> GAMGSYKDNIRHGVCWIYYPDGGSLVGEVNEDGEMTGEKIAYVYPDE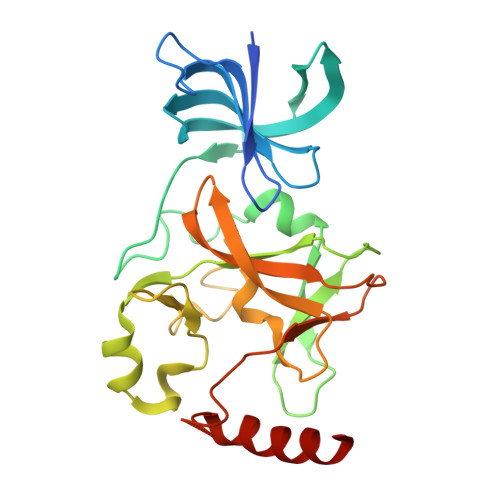RTALYGKFIDGEMIEGKLATLMSTEEGRPHFELMPGNSVYHFDKSTSSCISTNALLPDPYESERVYVAESLISSAGEGLFSKVAVGPNTVMSFYNGVRITHQEVDSRDWALNGATLSLDEETVIDVPEPYNHVSKYCASLGHKANHSFTPNCIYDMFVHPRFGPIKCIRTLRAVEADEELTVAYGYDHSPPGKSGPEAPEWYQVELKAFQATQQK>LYFQGHMQLSRKGLDAIKFFEGLELEAYEDSAGIPTIGYGTIRIDGKPVKMGMKITAEQAEQYLLADVEKFVAAVN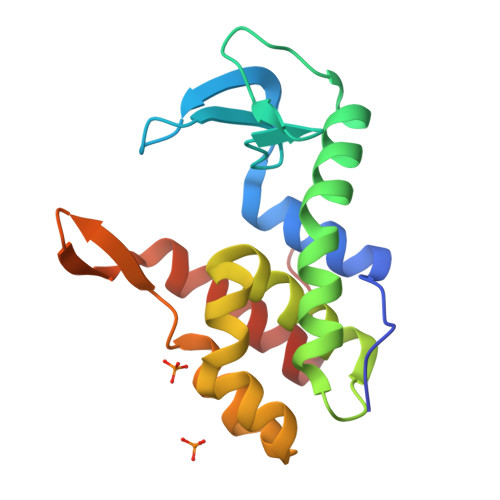KAIKVPTTQNEFDALVSETYNIGITAMQDSTFIKRHNAGNKVGCAEAMQWWNKVTVKGKKVTSNGLKNRRRMEADIYLDSVYPK[2x]>MTEQPAVAAPYDVLFEPVQIGPFTTKNRFYQVPHCNGMGYRDPSAQASMRKIKAEGGWSAVCTEQVEIHATSDIAPFIELRIWDDQDLPALKRIADAIHEGGGLAGIELAHNGMNAPNQLSRETPLGPGHLPVAPDTIAPIQARAMTKQDIDDLRRWHRNAVRRSIEAGYDIVYVYGAHGYSGVHHFLSKRYNQRTDEYGGSLENRMRLLRELLEDTLDECAGRAAVACRITVEEEIDGGITREDIEGVLRELGELPDLWDFAMGSWEGDSVTSRFAPEGRQEEFVAGLKKLTTKPVVGVGRFTSPDAMVRQIKAGILDLIGAAR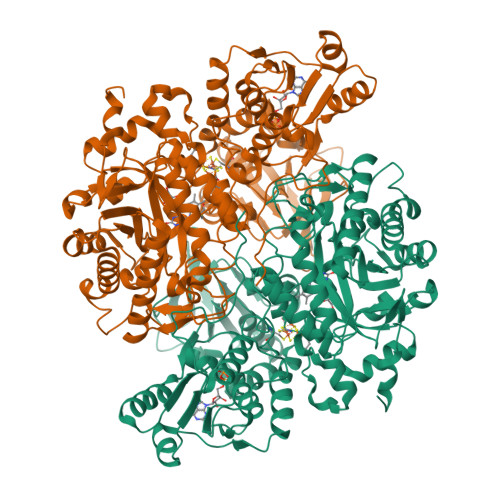PSIADPFLPNKIRDGRLNLIRECIGCNICVSGDLTMSPIRCTQNPSMGEEWRRGWHPERIRAKESDARVLVVGAGPSGLEAARALGVRGYDVVLAEAGRDLGGRVTQESALPGLSAWGRVKEYREAVLAELPNVEIYRESPMTGDDIVEFGFEHVITATGATWRTDGVARFHTTALPIAEGMQVLGPDDLFAGRLPDGKKVVVYDDDHYYLGGVVAELLAQKGYEVSIVTPGAQVSSWTNNTFEVNRIQRRLIENGVARVTDHAVVAVGAGGVTVRDTYASIERELECDAVVMVTARLPREELYLDLVARRDAGEIASVRGIGDAWAPGTIAAAVWSGRRAAEEFDAVLPSNDEVPFRREVTQLA[2x]> AQLTAQQRLLADQIISIFANNTPELQYGYAEVLDDGRGITAGRAGFTSATGDMLEVIQRYSRLRPDNILVPFLPRLQQLAASEDGSIEGLQGLPQRWADASQNPVFRQVQDDVVDELYFQPAMERAAELGAQMPLT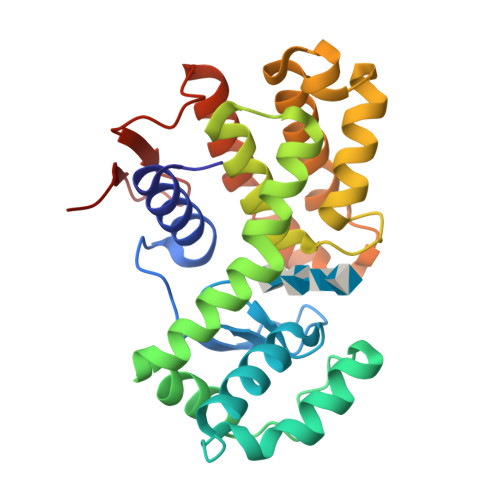LLALYDAIIQHGEGDDGDGLPAMIARTTAKVNGIPAEGVDERRWLKTFLKIRKQVLRHPANLETEDEWSESTGRVDSLMKLLKQGNTDLHPPIRISTWGDVFILPIR Recently, a shortened Dscam (sDscam) gene family with tandemly arrayed 5′ cassettes in Chelicerata species has been identified, which encodes ∼50–100 isoforms. Chelicerata sDscams could be classified into two subfamilies, sDscamα and sDscamβ, containing one and two variable Ig domains, respectively. Crystal structures and cell aggregation assays demonstrated that both α and β subfamilies of sDscam used Ig1 for the isoform-specific trans recognition in a hand-in-hand manner. Furthermore, the cis interactions were established by the three FNIII domains of sDscam, which assemble into a cross fold with a kink between FNIII2 and FNIII3.

We found that FNIII2 alone but not FNIII1 or FNIII3 could promote cKIT tyrosine phosphorylation, suggesting the essential role of FNIII2 domain in mediating sDscam cis interactions. The gel-filtration analysis supported our observations in the crystal structures: Ig1 mediated the formation of trans homodimer and all the three FNIII domains were involved in the cis interactions.

>GASPPSPPRGIKVSEVTTRTARLSWQSPYGNGDNTVVTYIVRYWRDEESRSQLHQLTFQVTSANLKDLHPGTSYAVQILAENDVGASIPSRLVQFRTIEE[2x]>SVTEFLKPRLVDIEQVSSTHAKVTLEPLERGFGHTLGNALRRILLSSMPGCAVTEVEIDGVLHEYSTKEGVQEDILEILLNLKGLAVRVQGKDEVILTLNKSGIGPVTAADITHDGDVEIVKPQHVICHLTDENASISMRIKVQRGRGYVPASTRIHSEEDERPIGRLLVDACYSPVERIAYNVEAARVEQRTDLDKLVIEMETNGTIDPEEAIRRAATILAEQLEAFVDLRDVRQPEVKEEKPEFDPILLRPVDDLELTVRSANCLKAEAIHYIGDLVQRTEVELLKTPNLGKKSLTEIKDVLASRGLSLGMRLENWPPA[2x];> MVYSYTEKKRIRKDFGKRPQVLDVPYLLSIQLDSFQKFIEQDPEGQYGLEAAFRSVFPIQSYSGNSELQYVSYRLGEPVFDVQECQIRGVTYSAPLRVKLRLVIYEREAPEGTVKDIKEQEVYMGEIPLMTDNGTFVINGTERVIVSQLHRSPGVFFDSDKGKTHSSGKVLYNARIIPYRGSWLDFEFDPKDNLFVRIDRRRKLPATIILRALNYTTEQILDLFFEKVIFEIRDNKLQMELVPERLRGETASFDIEANGKVYVEKGRRITARHIRQLEKDDVKLIEVPVEYIAGKVVAKDYIDESTGELICAANMELSLDLLAKLSQSGHKRIETLFTNDLDHGPYISETLRVDPTNDRLSALVEIYRMMRPGEPPTREAAESLFENLFFSEDRYDLSAVGRMKFNRSLLREEIEGSGILSKDDIIDVMKKLIDIRNGKGEVDDIDHLGNRRIRSVGEMAENQFRVGLVRVERAVKERLSLGDLDTLMPQDMINAKPISAAVKEFFGSSQLSQFMDQNNPLSEITHKRRISALGPGGLTRERAGFEVRDVHPTHYGRVCPIETPEGPNIGLINSLSVYAQTNEYGFLETPYRKVTDGVVTDEIHYLSAIEEGNYVIAQANSNLDEEGHFVEDLVTCRSKGESSLFSRDQVDYMDVSTQQVVSVGASLIPFLEHDDANRALMGANMQRQAVPTLRADKPLVGTGMERAVAVDSGVTAVAKRGGVVQYVDASRIVIKVNEDEMYPGEAGIDIYNLTKYTRSNQNTCINQMPCVSLGEPVERGDVLADGPSTDLGELALGQNMRVAFMPWNGYNFEDSILVSERVVQEDRFTTIHIQELACVSRDTKLGPEEITADIPNVGEAALSKLDESGIVYIGAEVTGGDILVGKVTPKGETQLTPEEKLLRAIFGEKASDVKDSSLRVPNGVSGTVIDVQVFTRDGVEKDKRALEIEEMQLKQAKKDLSEELQILEAGLFSRIRAVLVAGGVEAEKLDKLPRDRWLELGLTDEEKQNQLEQLAEQYDELKHEFEKKLEAKRRKITQGDDLAPGVLKIVKVYLAVKRRIQPGDKMAGRHGNKGVISKINPIEDMPYDENGTPVDIVLNPLGVPSRMNIGQILETHLGMAAKGIGDKINAMLKQQQEVAKLREFIQRAYDLGADVRQKVDLSTFSDEEVMRLAENLRKGMPIATPVFDGAKEAEIKELLKLGDLPTSGQIRLYDGRTGEQFERPVTVGYMYMLKLNHLVDDKMHARSTGSYSLVTQQPLGGKAQFGGQRFGEMEVWALEAYGAAYTLQEMLTVKSDDVNGRTKMYKNIVDGNHQMEPGMPESFNVLLKEIRSLGINIELED;> LLKFLKAQTKTEEFDAIKIALASPDMIRSWSFGEVKKPETINYRTFKPERDGLFCARIFGPVKDYECLCGKYKRLKHRGVICEKCGVEVTQTKVRRERMGHIELASPTAHIWFLKSLPSRIGLLLDMPLRDIERVLYFESYVVIEGGMTNLERQQILTEEQYLDALEEFGDEFDAKMGAEAIQALLKSMDLEQECEQLREELNETNSETKRKKLTKRIKLLEAFVQSGNKPEWMILTVLPVLPPDLRPLVPLDGGRFATSDLNDLYRRVINRNNRLKRLLDLAAPDIIVRNEKRMLQEAVDALLDNGRRGRAITGSNKRPLKSLADMIKGKQGRFRQNLLGKRVDYSGRSVITVGPYLRLHQCGLPKKMALELFKPFIYGKLELRGLATTIKAAKKMVEREEAVVWDILDEVIREHPVLLNRAPTLHRLGIQAFEPVLIEGKAIQLHPLVCAAYNADFDGDQMAVHVPLTLEAQLEARALMMSTNNILSPANGEPIIVPSQDVVLGLYYMTRDCVNAKGEGMVLTGPKEAERLYRSGLASLHARVKVRITEYEKDANGELVAKTSLKDTTVGRAILWMIVPKGLPYSIVNQALGKKAISKMLNTCYRILGLKPTVIFADQIMYTGFAYAARSGASVGIDDMVIPEKKHEIISEAEAEVAEIQEQFQSGLVTAGERYNKVIDIWAAANDRVSKAMMDNLQTETVINRDGQEEKQVSFNSIYMMADSGARGSAAQIRQLAGMRGLMAKPDGSIIETPITANFREGLNVLQYFISTHGARKGLADTALKTANSGYLTRRLVDVAQDLVVTEDDCGTHEGIMMTPVIEGGDVKEPLRDRVLGRVTAEDVLKPGTADILVPRNTLLHEQWCDLLEENSVDAVKVRSVVSCDTDFGVCAHCYGRDLARGHIINKGEAIGVIAAQSIGEPGTQLTMRTFHIGGAASRAAAESSIQVKNKGSIKLSNVKSVVNSSGKLVITSRNTELKLIDEFGRTKESYKVPYGAVLAKGDGEQVAGGETVANWDPHTMPVITEVSGFVRFTDMIDGQTITRQTDELTGLSSLVVLDSAERTAGGKDLRPALKIVDAQGNDVLIPGTDMPAQYFLPGKAIVQLEDGVQISSGDTLARIPQESGGTKDITGGLPRVADLFEARRPKEPAILAEISGIVSFGKETKGKRRLVITPVDGSDPYEEMIPKWRQLNVFEGERVERGDVISDGPEAPHDILRLRGVHAVTRYIVNEVQDVYRLQGVKINDKHIEVIVRQMLRKATIVNAGSSDFLEGEQVEYSRVKIANRELEANGKVGATYSRDLLGITKASLATESFISAASFQETTRVLTEAAVAGKRDELRGLKENVIVGRLIPAGTGYAYHQDRMRRRAAG;> ARVTVQDAVEKIGNRFDLVLVAARRARQMQVGGKDPLVPEENDKTTVIALREIEEGLINNQILDVRERQEQQEQ;> TAGTPSGNGVDYQDDELPVYQGETTQSLQDYLMWQVELTPFTDTDRAIATSIVDAVDDTGYLTIQIEDIVDSIGDDEIGLEEVEAVLKRIQRFDPVGVAAKDLRDCLLIQLSQFAKETPWLEEARLIISDHLDLLANHDFRTLMRVTRLKEEVLKEAVNLIQSLDPRPGQSIQTGEPEYVIPDVLVRKVNDRWVVELNSDSRWLIKSLESANDTLLRVSRCIVEQQQAFFEQGEEYMKPMVLADIAQAVEMHESTISRVTTQKYLHSPRGIFELKYFFSSHVNTEGGGEASSTAIRALVKKLIAAENPAKPLSDSKLTSMLSEQGIMVARRTVAKYRESLSIPPSNQ

Transcription initiation in bacteria involves the recruitment of RNAP by sigma factors (σ) to promoter regions located upstream from the transcription start site (TSS, position +1). In approximately 60% of bacteria, a major variant σ factor, σ54, forms a class of its own, lacking structural and sequence similarity to σ70. In σ54-mediated transcription initiation, σ54 recruits RNAP to genes responsible for regulating a variety of stress responses, including nutrient depletion, membrane stress, antibiotic exposure, and biofilm formation. In this study, we used single-particle cryo-electron microscopy (cryoEM) to determine the structures of initial transcribing complexes of increasing RNA lengths from 5 nt to 9 nt, which allow us to propose a mechanism of RNAP promoter escape in the σ54 system.

However, at 7 nt RNA, the RII-finger adapts a different conformation, to accommodate for the growing DNA–RNA hybrid and prevent steric clashes. The tip of the RII-finger is coiled backward by 9.5 Å, as measured from the Cα atoms of the tip of the RII-finger (Middle). In RPitc-7nt, the folded back RII tip is stabilized by interactions between Y112 of RII and V253 of β′, P110 with the DNA–RNA bases (Right). In addition, P110 and Y112, observed in 5 to 7nt complexes, were also not resolved, indicating that these interactions are no longer stably maintained. These results suggest that the folded-back conformation of the RII-finger observed in 7 nt complex is stabilized by specific hydrophobic interactions and therefore likely represents a kinetic barrier during initial transcription. Taken together, data presented here suggest that RNA extension to 7 nt causes the folding back of the RII-finger, which is stabilized by specific interactions between RNA, DNA, and RII-finger. In RPitc-6nt and RPitc-7nt, the template strand (at −5 and −6 positions) is scrunched around the RII-finger and σ54 ELH, while the nontemplate strand scrunches around the ELH, resulting in poorly defined density. From 7 nt, ELH and upstream DNA become more flexible, indicating a global conformational change occurring within the transcription complex. In σ54, we observe RII-finger folding back when RNA length reaches 7 nt to accommodate the increasing DNA–RNA hybrid.> GAYSGAPKQ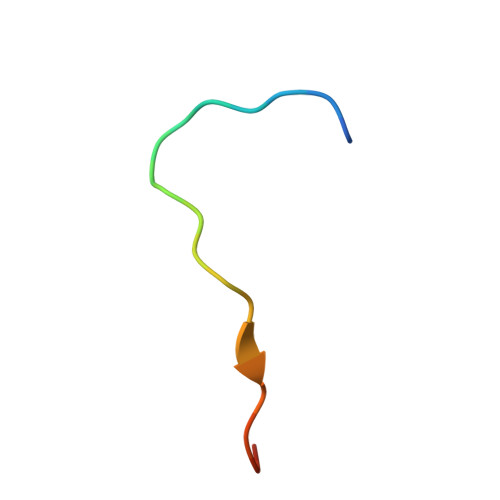VLKKPALRTATVQ> MSKGKLGEKISQFKIVEELKAKGLYAYFRPIQSKQDTEVKIDGRRVLMFGSNSYLGLTTDTRIIKAAQDALEKYGTGCAGSRFLNGTLDIHVELEEKLSAYVGKEAAILFSTGFQSNLGPLSCLMGRNDYILLDERDHASIIDGSRLSFSKVIKYGHNNMEDLRAKLSRLPEDSAKLICTDGIFSMEGDIVNLPELTSIANEFDAAVMVDDAHSLGVIGHKGAGTASHFGLNDDVDLIMGTFSKSLASLGGFVAGDADVIDFLKHNARSVMFSASMTPASVASTLKALEIIQNEPEHIEKLWKNTDYAKAQLLDHGFDLGATESPILPIFIRSNEKTFWVTKMLQDDGVFVNPVVSPAVPAEESLIRFSLMATHTYDQIDEAIEKMVKVFKQAEVETLI

pmcSerine palmitoyltransferase (SPT) is a key enzyme of sphingolipid biosynthesis and catalyzes the pyridoxal-5′-phosphate (PLP)-dependent decarboxylative condensation reaction between l-serine and palmitoyl-CoA to form 3-ketodihydrosphingosine (KDS), also called a long-chain base (LCB), as a common precursor of all sphingolipids. Bacterial SPTs from sphingolipid-containing bacteria such as Sphingomonas paucimobilis, which is rich in glycosphingolipids, and Sphingobacterium multivorum, which is rich in phosphosphingolipids, function as a water-soluble homodimer enzyme and are useful as a prototypical model system of human SPT. Based on these enzymological and structural analyses, the synthesis of KDS from d-serine was explained as the result of the slow racemization to l-serine, followed by the reaction with palmitoyl-CoA, and SPT would not catalyze the direct condensation between d-serine and palmitoyl-CoA.

To further study the substrate recognition mechanism and the mechanism of the KDS production from d-serine by SPT, we tried to prepare the crystal of SPT complexed with d-serine by a soaking experiment. The SPT crystals were soaked in a solution supplemented with 190 mM d-serine for 10 min and subjected to X-ray structure analysis. This d-serine–soaked crystal diffracted to 1.65 Å resolution, and the diffraction data were indexed in the tetragonal space group P41212 with unit cell parameters, a = b = 61.0 Å, c = 207.3 Å, α = β = γ = 90°. The crystal structure was determined at a resolution of 1.65 Å and refined to Rwork and Rfree values of 0.149 and 0.184, respectively, with a Cruickshank diffraction-component precision index of 0.0921 Å. The final model contained 394 amino acid residues, one PLP, 419 water molecules, and seven ethylene glycol molecules per monomer. Unexpectedly, a model of the PLP–l-serine external aldimine was well assigned at the occupancy of 1 to this electron density map. The amount of l-serine in the commercial d-serine sample was below the detection limit, but the possibility that the binding affinity of d-serine to SPT in crystal is so low that even a trace amount of contaminating l-serine yields the SPT–l-serine binary complex cannot be ruled out. The reason why the electron density of the PLP–d-serine external aldimine was not detected in the d-serine–soaked SPT crystal is explained as follows: d-serine was converted to l-serine by SPT in the crystal during the soaking treatment, and the l-serine with more than 20 times higher affinity to SPT than d-serine remained in the active site, resulting in the structure of the l-serine complex of SPT.> MATTTNILHDVVRDQSMVNYVSNRDRPLYFKRPLVPQMTDIPLHISRPPVDQQVDYQTMQMQQNATIVEAPTKDAFVQTDYRESETQTDPYTPKCFVRDGDHPEVMELKDYKYGKGLPASIEELEQIELNREKVWFENSLPPISDEASFNLRRKLMEEQELREWSKKENEIKKFQNEKLYLLQQALIEREKEVEDKSQERIEEIRQQKTEHKNRQIAKIQRKKIKIDRKMTKSRKMQGKETLKRDIIEDYANFASRVYAGITHEGLSLDKIANKYEVQPLALGNYEMLQALHEGIRPREFETRVNLKKEIKEIEKNYTRLENYHRGELKKAQDEINGVHEQSKAQQKQEGNNFSYRNFENKIRPATPTWKYDTDFNISPSLITEIQEYRGPNGVQLMQAADKREEAVLLLQRLLRGRTT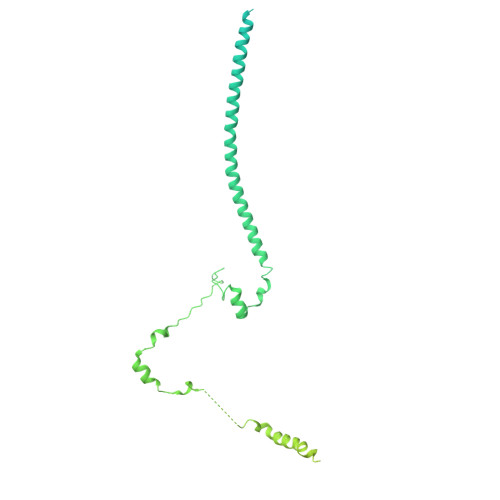QNIMYEGKKKRTALIEELLTVAQIENLEEDKAEEVLMQQHEEKVKNAVLESIQGEVIAETMDELSKELLRIKQERKIQQMVEIAEKDRRIREIEEAGKRQAEEILRDREDVLHNQLIRVHQGTVDTYLDWLMSNALEQSSARQATIMTNLRKAKFNLPLEDFERKYNNNQTLIKDLVHSFLIPNVQRSKLKKQIQLEEKRFSEAAKRSLQQTITRASNKHANVQN>SMLIDLIT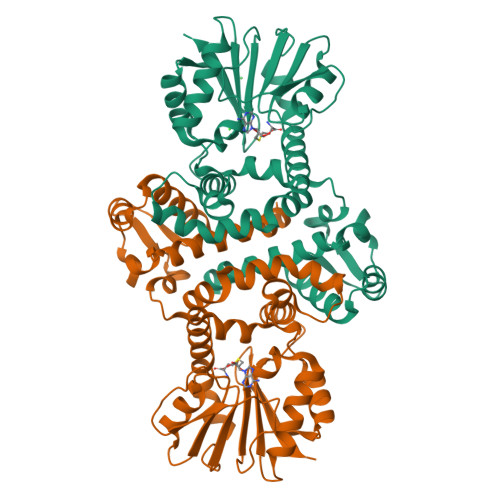SYRKTAAIYTFVDAGLSIHFKNGDYVDINKLASQYGIDYSRLNRLCDFLIEIGVLVSSDHGVALSEECSALADPNSVEFLTVKYEINSEHWDSWLMYPKSLLENNGKSAFEMVHGKSFFEHLDSNKGLKSDFDALMSKYTNKIIKELLVIYDFDKHNRILDLGGGDGELLIRISEQVKGKDYTVLDRYNEVPISEGINFIKGDFFKPIPTGYDLYILKNVLHNWPDNDAISILKNCREAMDNNATLLIITLMKKPQSLVVKSVDILMDMLFSAKQRYLSEFEDIANQAGLVIRHYKDLDEIFSLIELKVK[8x]>[4x]SNAMLVIEDVRAYEVLDSRGNPTVKAEVTLSDGSVGAAIVPSGASTGSKEALELRDNDERFGGKGVLKAVANVNETIADEILGLDAFNQTQLDDTLRELDGTNNYSNLGANATLGVSMATARAAAAALGMPLYRYLGGANASILPVPMCNIINGGAHANNNVDFQEFMIMPFGFTSFKEALRSVCEIYAILKKELANSGHSTALGDEGGFAPNLANNTEPIDLLMTCIKKA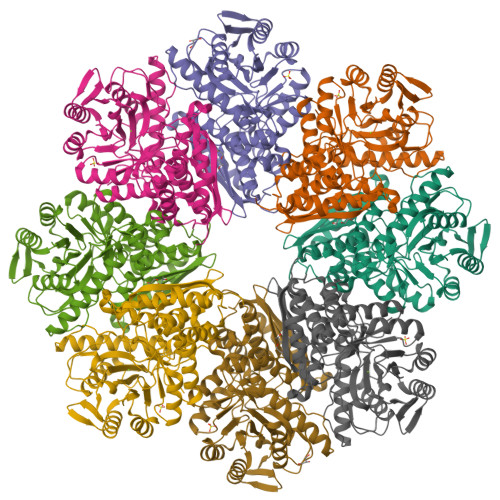GYENRVKIALDVASTEFFKDGKYHMEGKAFSSEALIERYVELCAKYPICSIEDGLAENDFEGWIKLTEKLGNKIQLVGDDLFVTNEDILREGIIKKMANAVLIKPNQIGTITQTMRTVRLAQRNNYKCVMSHRSGESEDAFIADFAVALNTGQIKTGALARGERTAKYNRLLEIEFESDEYLGEKL>[2x]DQCIVDDITYNVQDTFHKKHEEGHMLNCTCFGQGRGRWKCDPVDQCQDS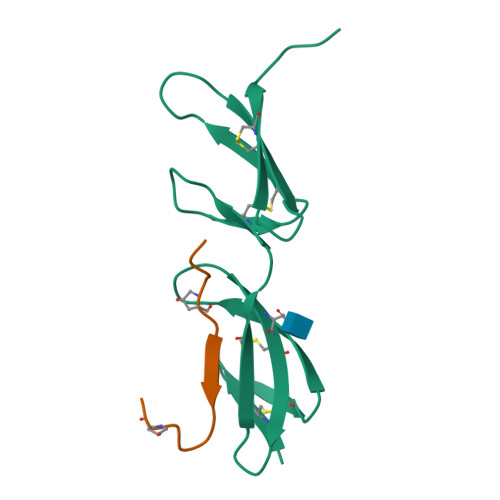ETGTFYQIGDSWEKYVHGVRYQCYCYGRGIGEWHCQPLQTYPSS;>GQRGVVGLPGQRGERGFPGLPGY[2x]> GPPGPKGPKGDP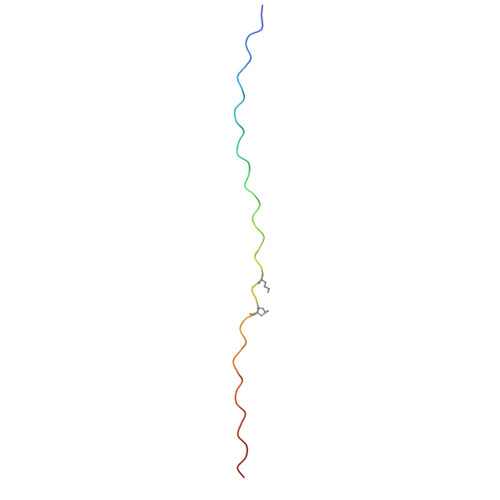GDPGPPGARGQAGVLGFPGPPGPKGPKGDPGDPG> MITINNDPFQEYQKDFAYCESIIKKNSKSFYLAFSQLPKRKAQSVYAVYAFCRRADDLIDRDNNQAGLRQLERQLLDFNEGKVPNDPVWRALSVVFDNFPMVTAPFFDMLTGQRKDADFKQPETRKDLEEYCYYVAGSVGLMLLPLLT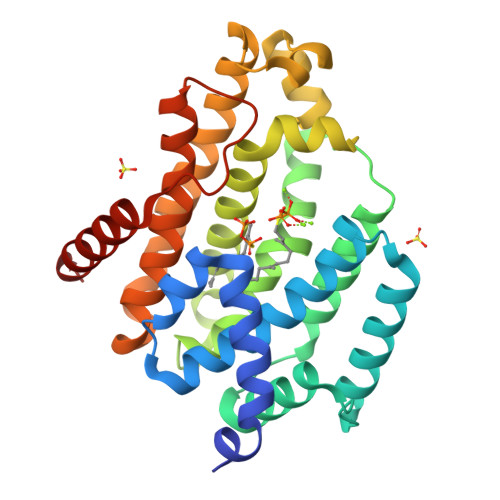ERPADIVVPAKKLGEAMQLTNILRDVGEDYQMGRIYLTKEDMTRFGVATTMLKEKQAQTQLVALWESLAKQAENLYEESFEMFPLITEDCRQALASAAFIYREQLNIVRKQHYSLFDNKNKVSHYRKVQLLKEVKSYLKSY> MLSKTILDKLNHQVNFEAASAHLYLQMSAWLLTQSLDSTAAFFRAHAEEEKAHMMKLFDYINETGSLALIGEVATPAPEWKSHIELLEAAYNHELAITQSINDLVDTALREKDYSTFQFLQWYVAEQHEEEYLFSSMLHKARII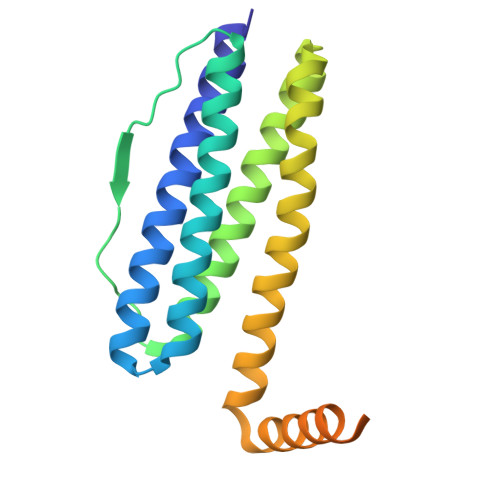DTMDGRALFRFDEEVRKSVLHHEHHQQKPMFLQVGPAPKHHDGHDGLHAHQHSSHWSGH>[4x]GSVWCRHCGATSAGLRCEWQNNYTQCAPCASLSSCP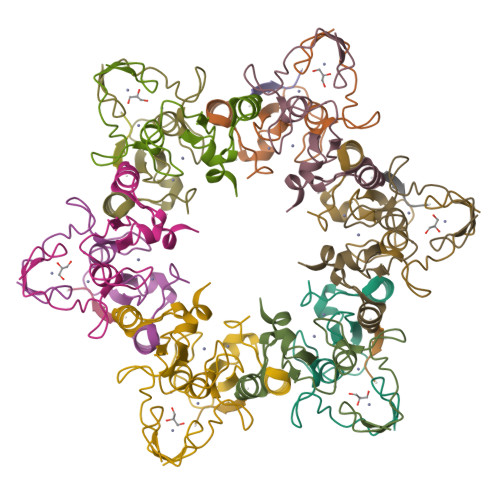VCYRNYREEDLILQCRQCDRWMHAVCQNLNTEEEVENVADIGFDCSMCRPYMPASN;>SGRGKGGKGLGKGGAKRHRK[2x]> GCCSHPACAGNNQHIC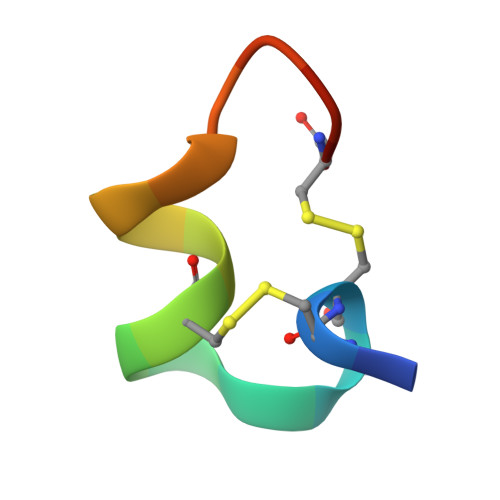X In addition, mamba venoms contain aminergic toxins that recognize various bioaminergic receptors. Aminergic toxins belong to the three-finger fold toxin (3FT) superfamily, a structural fold known to support a large diversity of biological functions. Despite sequence identities that vary from 70 to 98%, aminergic toxins display highly variable pharmacological profiles. Here, we use the ancestral protein resurrection methodology on the aminergic toxin group in order to pinpoint the functional substitutions which may have occurred during their evolution and use them for molecular engineering.

In order to visually understand the evolution of the AncTxs, the crystallographic structure of AncTx1 (variant W28R-I38S) was solved. As it might have been expected, the structure was rigid, except at the tips of the three loops. AncTx1W28R-I38S represents well AncTx1 as the two mutations on loop 2 do not perturb the structure, as can be verified by comparing AncTx1W28R-I38S with MT2. Loop 1 is more susceptible to backbone variations, and both MT7 and MT2 are subjected to a large kink at the tip of this loop. The selectivity of AncTx1 is characterized by a slightly higher affinity for α1A and a much lower one for the α1B and α2C receptors, relative to ρ-Da1a. Having recognized that the substitution (I38S) in AncTx3 affects α1D binding and that (W28R) increases α1B and α2C binding, the appropriate substitutions were integrated stepwise in AncTx1 to boost its selectivity. The pKi values for the AncTx1 double variant W28R-I38S were calculated to be 8.59, 6.41, 3.71 and 4.85 toward α1A, α1B, α1D and α2C respectively showing that despite an impressive loss in α1D affinity (3.71 vs. 6.58 for AncTx1), the selectivity of this variant suffered from a large pKi gain toward α1B (6.41 vs. 4.75 for AncTx1 I38S). We increased the affinity of AncTx1 for the α1B, α1D or α2C receptors with just two variants, unfortunately without achieving our primary goal to improve selectivity. Epistasis, a phenomenon already stated as important in protein evolution may have been the cause as revealed by other ancestral resurrection studies. Indeed, the functional effects of a substitution could depend on its surrounding context or sequence background.

> LTCVKSKSIFGVTTEDCPDGQNLCFKRRHYIVPKMYDSTRGCAATCPIAENRDVIHCCGTDKCNE>[2x]MKFTVEREHLLKPLQQVSGPLGGRPTLPILGNLLLQVADGTLSLTGTDLEMEMVARVALVQPHEPGATTVPARKFFDICRGLPEGAE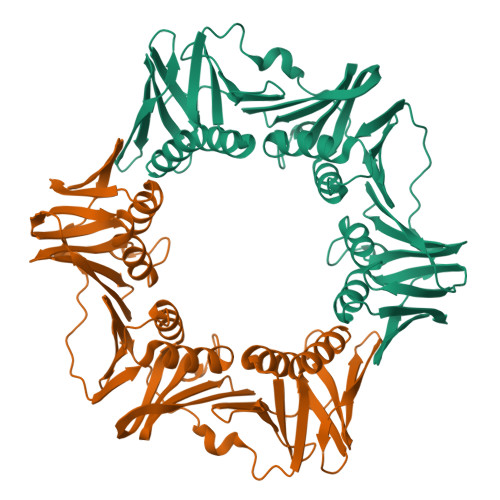IAVQLEGERMLVRSGCSRFSLSTLPAADFPNLDDWQSEVEFTLPQATMKRLIEATQFSMAHQDVRYYLNGMLFETEGEELRTVATDGHRLAVCSMPIGQSLPSHSVIVPRKGVIELMRMLDGGDNPLRVQIGSNNIRAHVGDFIFTSKLVDGRFPDYRRVLPKNPDKHLEAGSDLLKQAFARAAILSNEKFRGVRLYVSENQLKITANNPEQEEAEECLDVTYSGAEMEIGFNVSYVLDVLNALKSENVRMMLTDSVSSVQIEDAASQSAAYVVMPMRL>MKVNNTIVVSIGQAGNQIAASFWKTVCLEHGIDPLTGQTAPGVAPRGNWSSFFSKLGESSSGSYVPRAIMVDLEPSVIDNVKATSGSLFNPANLISRTEGAGGNFAVGYLGAGREVLPEVMSRLDYEIDKCDNVGGIIVLHAIGGGTGSGFGALLIESLKEKYGEIPVLSCAVLPSPQVSSVVTEPYNTVFALNTLRRSADACLIFDNEALFDLAHRKWNIESPTVDDLNLLITEALAGITASMRFSGFLTVEISLRELLTNLVPQPSLHFLMCAFAPLTPPDRSKFEELGIEEMIKSLFDNGSVFAACSPMEGRFLSTAVLYRGIMEDKPLADAALAAMREKLPLTYWIPTAFKIGYVEQPGISHRKSMVLLANNTEIARVLDRICHNFDKLWQRKAFANWYLNEGMSEEQINVLRASAQELVQSYQVAEESGAKAKVQDSAGDTGMRAAAAGVSDDARGSMSLRDLVDRRR[2x];> SDKIIHLTDDSFDTDVLKADGAILVDFWAEWCGPCKMIAPILDEIADEYQGKLTVAKLNIDQNPGTAPKYGIRGIPTLLLFKNGEVAATKVGALSKGQL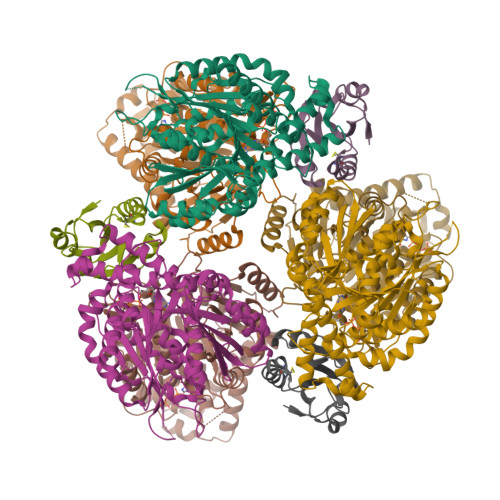KEFLDANLA> PISPIETVPVKLKPGMDGPKVKQWPLTEEKIKALVEICTEMEKEGKISKIGPENPYNTPVFAIKKKDSTKWRKLVDFRELNKRTQDFWEVQLGIPHPAGLKKKKSVTVLDVGDAYFSVPLDEDFRKYTAFTIPSINNETPGIRYQYNVLPQGWKGSPAIFQSSMTKILEPFRKQNPDIVIYQYMDDLYVGSDLEIGQHRTKIEELRQHL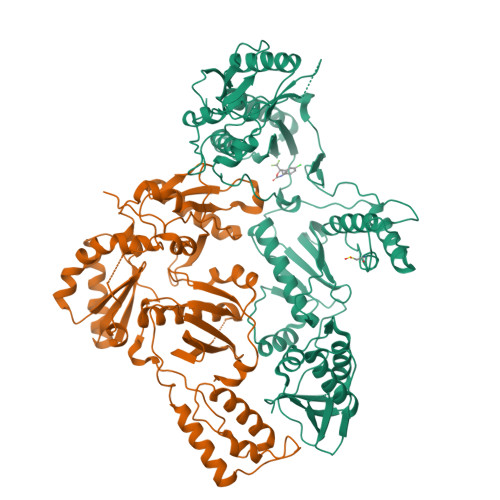LRWGLTTPDKKHQKEPPFLWMGYELHPDKWTVQPIVLPEKDSWTVNDIQKLVGKLNWASQIYPGIKVRQLCKLLRGTKALTEVIPLTEEAELELAENREILKEPVHGVYYDPSKDLIAEIQKQGQGQWTYQIYQEPFKNLKTGKYARMRGAHTNDVKQLTEAVQKITTESIVIWGKTPKFKLPIQKETWETWWTEYWQATWIPEWEFVNTPPLVKLWYQLEKEPIVGAETFYVDGAANRETKLGKAGYVTNRGRQKVVTLTDTTNQKTELQAIYLALQDSGLEVNIVTDSQYALGIIQAQPDQSESELVNQIIEQLIKKEKVYLAWVPAHKGIG;> PISPIETVPVKLKPGMDGPKVKQWPLTEEKIKALVEICTEMEKEGKISKIGPENPYNTPVFAIKKKDSTKWRKLVDFRELNKRTQDFWEVQLGIPHPAGLKKKKSVTVLDVGDAYFSVPLDEDFRKYTAFTIPSINNETPGIRYQYNVLPQGWKGSPAIFQSSMTKILEPFRKQNPDIVIYQYMDDLYVGSDLEIGQHRTKIEELRQHLLRWGLTTPDKKHQKEPPFLWMGYELHPDKWTVQPIVLPEKDSWTVNDIQKLVGKLNWASQIYPGIKVRQLCKLLRGTKALTEVIPLTEEAELELAENREILKEPVHGVYYDPSKDLIAEIQKQGQGQWTYQIYQEPFKNLKTGKYARMRGAHTNDVKQLTEAVQKITTESIVIWGKTPKFKLPIQKETWETWWTEYWQATWIPEWEFVNTPPLVKLWYQLEKEPIVGAETF>[2x]GFRGVEEKKSLEILLKDDRLDTEKLCTFSQRFPLPSMYRALVWKVLLGILPPHHESHAKVM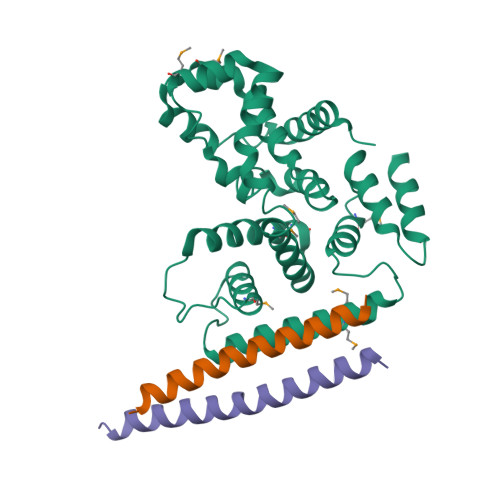MYRKEQYLDVLHALKVVRFVSDATPQAEVYLRMYQLESGKLPRSPSFPLEPDDEVFLAIAKAMEEMVEDSVDCYWITRRFVNQLNTKYRDSLPQLPKAFEQYLNLEDGRLLTHLRMCSAAPKLPYDLWFKRCFAGCLPESSLQRVWDKVVSGSCKILVFVAVEILLTFKIKVMALNSAEKITKFLENIPQDSSDAIVSKAIDLWHKHCGTPVHSS;>GGQLQAAESRYEAQKRITQVFELEILDLYGRLEKDGLLKKLEEEKAEAAEAAEER[4x]> MSKPNLEWLASLESKEAKSTVDSSDMDNDQKEGSDKSQQDEATEPEKKITATDVQIAIEEYARIRALTTTKDLPTDPEPGDTYHVNGVDWIYQEDGGWVTMQGIYGHEHFD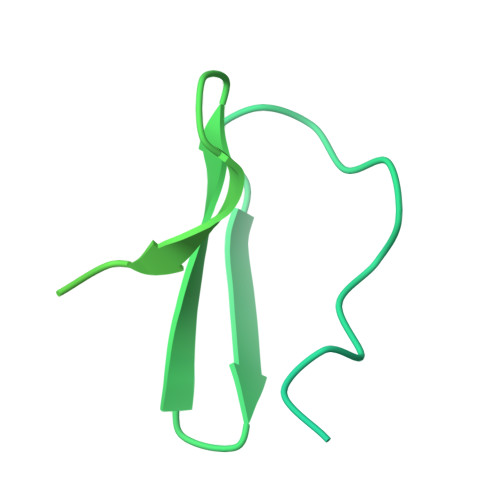ENGLNIEASGIDQKSGATKRYVVTGYNAQTNPAAMPGDNLTECVILMQNGLVPEVGVNGLTADCLLKIVKDLFEGYQAGPFACEENQVVINSMDRALSAIHQRLVRRKEQGTEGTYSGN> IVCHT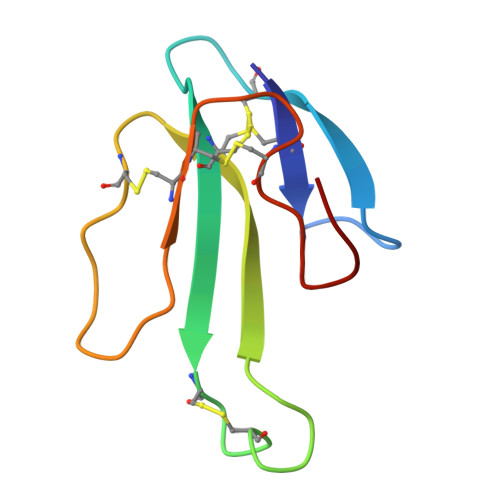TATSPISAVTCPPGENLCYRKMWCDVFCSSRGKVVELGCAATCPSKKPYEEVTCCSTDKCNPHPKQRPG> MSSNRVLDLFKPFESFLPEVIAPERKVPYNQKLIWTGVSLLIFLILGQIPLYGIVSSETSDPLYWLRAMLASN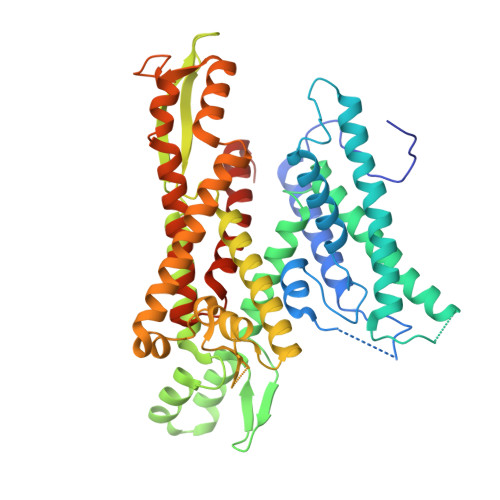RGTLLELGVSPIITSSMIFQFLQGTQLLQIRPESKQDRELFQIAQKVCAIILILGQALVVVMTGNYGAPSDLGLPICLLLIFQLMFASLIVMLLDELLSKGYGLGSGISLFTATNIAEQIFWRAFAPTTVNSGRGKEFEGAVIAFFHLLAVRKDKKRALVEAFYRTNLPNMFQVLMTVAIFLFVLYLQGFRYELPIRSTKVRGQIGIYPIKLFYTSNTPIMLQSALTSNIFLISQILFQKYPTNPLIRLIGVWGIRPGTQGPQMALSGLAYYIQPLMSLSEALLDPIKTIVYITFVLGSCAVFSKTWIEISGTSPRDIAKQFKDQGMVINGKRETSIYRELKKIIPTAAAFGGATIGALSVGSDLLGTLGSGASILMATTTIYGYYEAAAKEGGFTKNLVPGFSDLM>[3x]MASIAKKRLAQERAEWRKDHPAGFSAKYSPMSDGKGLDIMKWICKIPGKKGGLWEGGEYPLTMEFT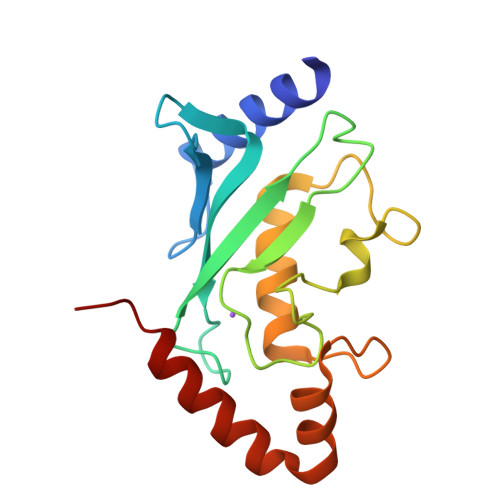EDYPSKPPKCKFTTVLFHPNIYPSGTVCLSILNEDEDWKPSITIKQILLGIQDLLDNPNPNSPAQAEPFLLYQQDRDSYEKKVKKQAIEFRPKD> MASMTGGQQMGRDEAGITGTWYN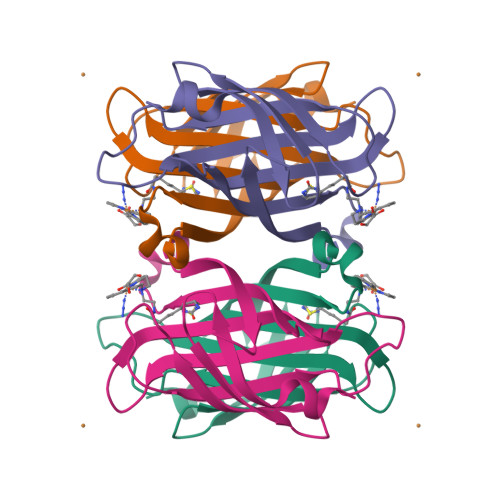QLGSTFIVTAGADGALTGTYESAVGNAESRYVLTGRYDSAPATDGSGTALGWTVAWKNNYRNAHSATTWSGQYVGGAEARINTQWLLTSGTTEANAWKSTLVGHDTFTKVKPSAASIDAAKKAGVNNGNPLDAVQQ> MRGIEITITMQSDWHVGTGMGRGELDSVVQRDGDNLPYIPGKTLTGILRDSCEQVALGLDNGQTRGLWHGWINFIFGDQPALAQGAIEPEPRPALIAIGSAHLDPKLKAAFQGKKQLQEAIAFMKPGVAIDAITGTAKKDFLRFEEVVRLGAKLTAEVELNLPDNLSETNKKVIAGILASGAKLTERLGGKRRRGNGRCELKFSGYSDQQIQWLKDNYQSVDQPPKYQQNKLQSAGDNPEQQPPWHIIPLTIKTLSPVVLPARTVGNVVECLDYIPGRYLLGYIHKTLGEYFDVSQAIAAGDLIITNATIKIDGKAGRATPFCLFGEKLDGGLGKGKGVYNRFQESEPDGIQLKGERGGYVGQFEQEQRNLPNTGKINSELFTHNTIQDDVQRPTSDVGGVYSYEAIIAGQTFVAELRLPDSLVKQITSKNKNWQAQLKATIRIGQSKKDQYGKIEVTSGNSADLPKPTGNNKTLSIWFLSDILLRGDRLNFNATPDDLKKYLENALDIKLKERSDNDLICIALRSQRTESWQVRWGLPRPSLVGWQAGSCLIYDIESGTVNAEKLQELMITGIGDRCTEGYGQIGFNDPLLSASLGKLTAKPKASNNQSQNSQSNPLPTNHPTQDYARLIEKAAWREAIQNKALALASSRAKREEILGIKIMGKDSQPTMTQLGGFRSVLKR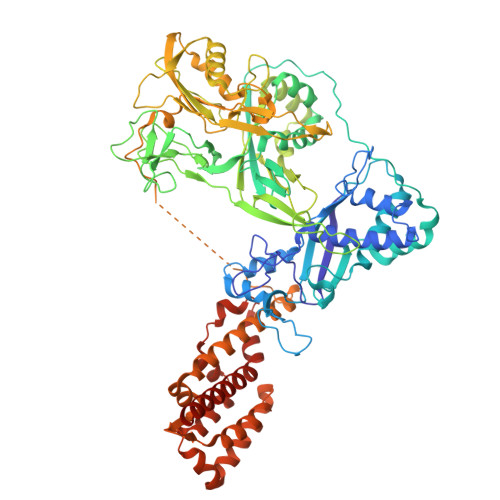LHSRNNRDIVTGYLTALEQVSNRKEKWSNTSQGLTKIRNLVTQENLIWNHLDIDFSPLTITQNGVNQLKSELWAEAVRTLVDAIIRGHKRDLEKAQENESNQQSQGAA> MDKVQYLTRSAIRRASTIEMPQQ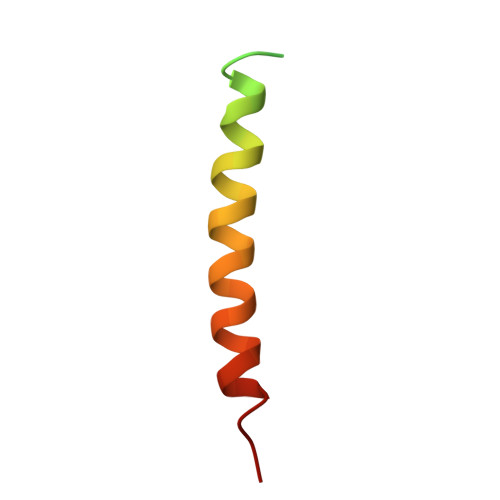ARQNLQNLFINFCLILICLLLICIIVM> GHMKIVLKIFHAGSLSVPFEEYEKMFEKEHPNVDVEREPAGSVACVRKIIDLGKKADILASADYSLIPQMMMPKYADWYVMFARNEIVLAYTDKSKYKDEINSTNWYKILQRPDVKIGFSNPNDDPCGYRTQMVLQLAELYYKDPTIYDNLVLKHSNIKVEENNGTYLILVPKELDVDTNKLFVRSKETDLLAPLEAGAFDYLFIYKSVANQHHLKYIELPKEINLGYYEYADTYKKVALKIIAKNKTI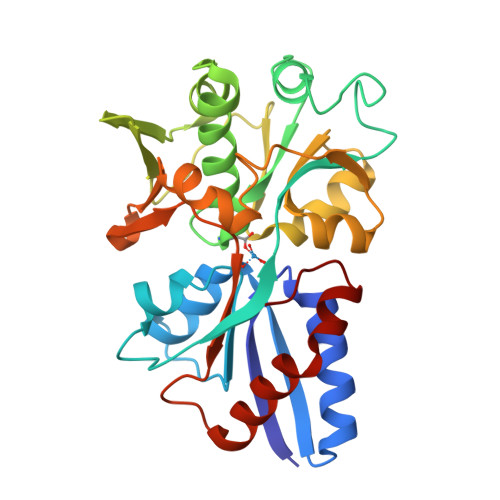NAKPIVYGMTVPTNAPHKKEAIEFVKFVLGHPEVLENNGQPAI> SENDSIELDDVANLMFYGEGQIGTNKQPFMFIFDTGSANLWVPSVNCDSIGC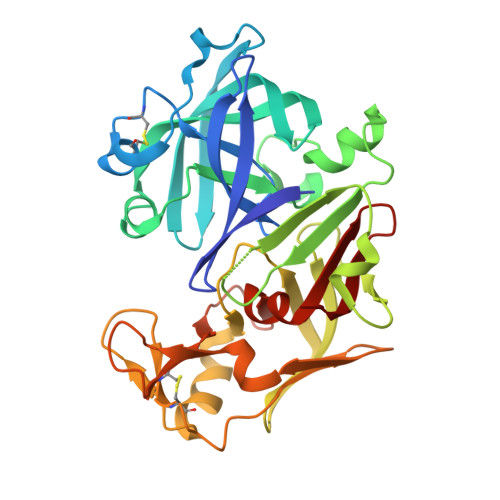STKHLYDASASKSYEKDGTKVEISYGSGTVRGYFSKDVISLGDLSLPYKFIEVTDADDLEPIYSGSEFDGILGLGWKDLSIGSIDPVVVELKKQNKIDNALFTFYLPVHDKHVGYLTIGGIESDFYEGPLTYEKLNHDLYWQIDLDIHFGKYVMQKANAVVDSGTSTITAPTSFLNKFFRDMNVIKVPFLPLYVTTCDNDDLPTLEFHSRNNKYTLEPEFYMDPLSDIDPALCMLYILPVDIDDNTFILGDPFMRKYFTVFDYEKESVGFAVAKNL> GUGCGACAAGAAGUUCAGGAAGGGAUUGAGGUGAAAGUCCUCCUCCCGAAUCGUUCAUGGGAGAGUCUAUCCAGACUUGCGUAGCGAGUAAUCGCUAGGUGAGAAGCUCUGGAGACAAUGUACCUGCCCUUCAAUUGGAGGUGCCAGGGCUAGGCUUUGUUCCUAUGGCUAGCGAAAGCGAAUACAGGUUAUUAGGCGUCGUGAAAACAAAACUCUUUCGACAUAAGGGAGAGGCUCGUAGAUGAGUUACCCUCCUUUUUAUGGGGUAACUGAACGAUCAAUAUCUACCGGCGUAGACUGUGAGCCUAAAGGAAACGAAUGAAAGUGUCCCUUCCUGGGAACUUGGUAAGCCCAAUAGACUCCCUCUGGGAAACCAGAGGAGGAGUAAGAGCAAUCUUACUUAUCGUCUAGUGGGUAAAAGACAUAAUAGGAAGCAAAUGCUUGGUUGUAACGAUCGAGAUAGAAUCUGUUGAUUUAAGCUGAAAGGCUGCAGACUUAUUAAAUGGGUGUUCUGCUGUAUGGCGUUCGCGCCUAAGCAGCAGAAUGCGUGAGCCGU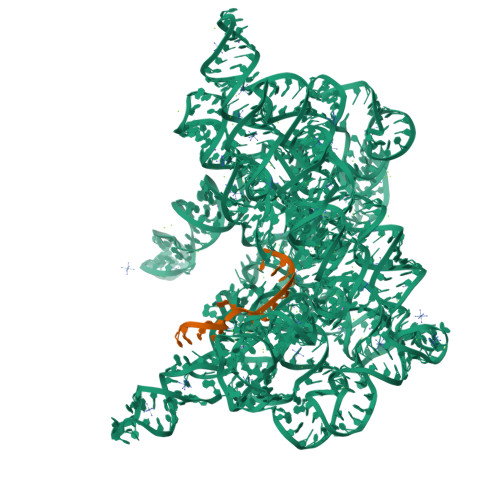GUGCGAUGAAAGUCGCAAGCACGGUUCUGAUGGGGGGAAAACGAGAGAUCGUCUACCUAUCCAAC;> UGUUUAUUAAAAAC> MNAHLANEVQYDLGHVPGRPSSLVHVIISSECLAAAGIPLAALMRGRPGLGTAANFQVEIQTRAHATGDCTPWCTAFAAYVPADAVGELLAPVVPAHPGLLPRASSAGGLFVSLPVVCDAQGVYDPYAVAALRLAWGSGASCARVILFSYDELVPPNTRYAADSTRIMRVCRHLCRYVALLGAAAPPAAKEAAAHLSMGLGESASPRPQPLARPHAGAPADPPIVGASDPPISPEEQLTAPGGDTTAAQDVSIAQENEEILALVQRAVQDVTRRHPVRARTGRAACGVASGLRQGALVHQAVSGGAMGAADADAVLAGLEPPGGGRFVAPVPHGPGGEDILNDVLTLTPGTAKPRSLVEWLDRGWEALAGGDRPDWLWSRRSISVVLRHHYGTKQRFVVVSYENSVAWGGRRARPPLLSSALATALTEACAAERVVRPHQLSPAGQAELLLRFPALEVPLRHPRPVLPPFDIAAEVAFTARIHLACLRALGQAIRAALQGGPRISQRLRYDFGPDQRAWLGEVTRRFPILLENLMRAVEGTAPDAFFHTAYALAVLAHLGGRGGRGR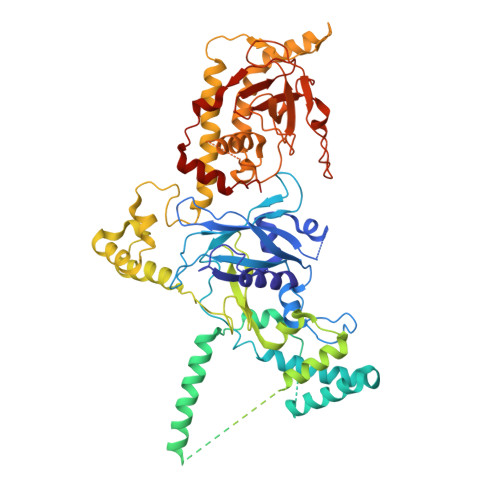RVVPLGDDLPARFADSDGHYVFDYYSTSGDTLRLNNRPIAVAMDGDVSKREQSKCRFMEAVPSTAPRRVCEQYLPGESYAYLCLGFNRRLCGIVVFPGGFAFTINIAAYLSLSDPVARAAVLRFCRKVSSGNGRSR> MYLTAVSTYFSYGLLFAFGQLRDFFRRFIDWWFTSNLQGYAPICLGHEDFYIRRLYHRIQ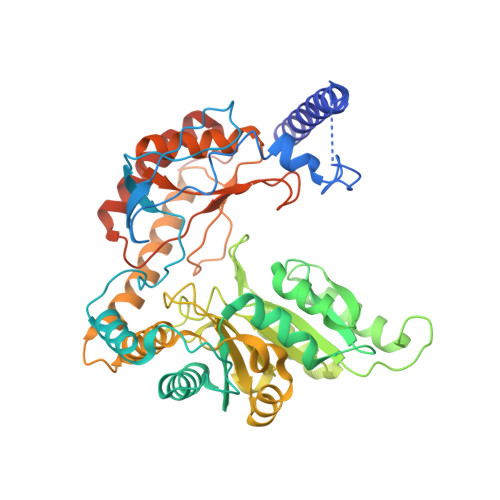DCFERPISSAPDAWFDVVERYSNDNNKTLKRTTKTSRCLNLGSYNYLGFGSFDEYCTPRVIESLKKFSASTCSSRVDAGTTSVHAELEECVTRFVGKPAAVVFGMGYATNSAIIPVLIGKGGLIISDSLNHSSIVNGARGSGATIRVFQHNTPSHLERVLREQIAEGQPRTHRPWKKIIVVVEGIYSMEGEICHLPEVVAICKKYKAYVYLDEAHSIGAIGKTGKGICELLGVDTADVDVMMGTFTKSFGSCGGYIAGSKELIQYLKHQCPAHLYATSIPTPSAQQIISAIKVILGEDGSNRGAQKLARIRENSNFFRAELQKMGFEVLGDNDSPVMPIMLYNPAKIPAFSRECLRQKVAVVVVGFPATPLLLARARICISASHSREDLIRALKVISKVGDLSGIKYFPAEPKKIEQSKNDIKLD> MSSQAFTSVHPNAATSDVNVTIDTFVAKLKRRQVQGSYAIALETLQLLMRFISAARWNHVNDLIEQIRDLGNSLEKAHPTAFSCGNVIRRILAVLRDEVEEDTMSTTVTSTSVAEPLISSMFNLLQKPEQPHQNRKNSSGSSSMKTKTDYRQVAIQGIKDLIDEIKNIDEGIQQIAIDLIHDHEILLTPTPDSKTVLKFLIT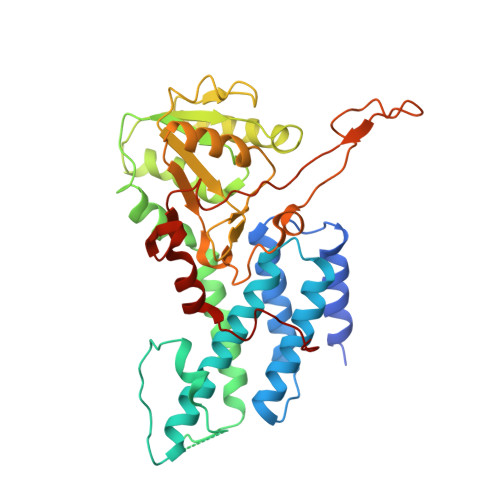ARERSNRTFTVLVTEGFPNNTKNAHEFAKKLAQHNIETLVVPDSAVFALMSRVGKVIIGTKAVFVNGGTISSNSGVSSVCECAREFRTPVFAVAGLYKLSPLYPFDVEKFVEFGGSQRILPRMDPRKRLDTVNQITDYVPPENIDIYITNVGGFNPSFIYRIAWDNYKQIDVHLDKNKA2-HYDROXYISONICOTINIC ACID N-OXIDE | C6 H5 N O4 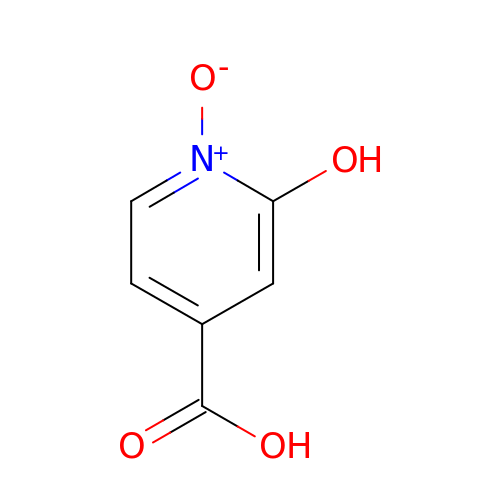| OFOAWMIVKVXKCO-UHFFFAOYSA-N>TFRMRIYERDDFRGQMSEITADCPSLQDRFHLTEVHSLN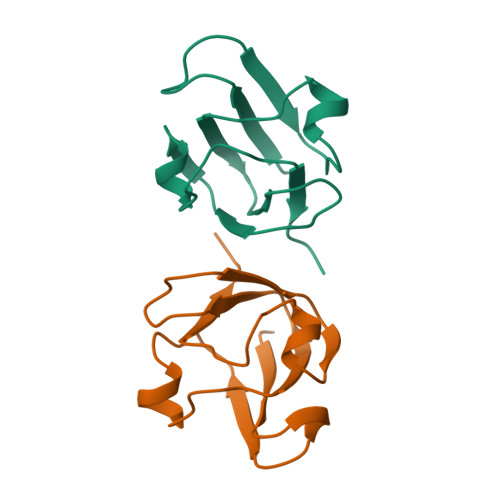VLEGSWVLYEMPSYRGRQYLLRPGEYRRYLDWGAMNAKVGSLRRVMD[2x]>[2x]TLQPTEAAYIAGFLDGDGSIYARLEPRPDYKDIKYQVRLAISFIQRKDKFPYLQDIYDQLGKRGILRKDRGDGIADYRIYGSTHLSIILPDLVPYLRIKKKQANRI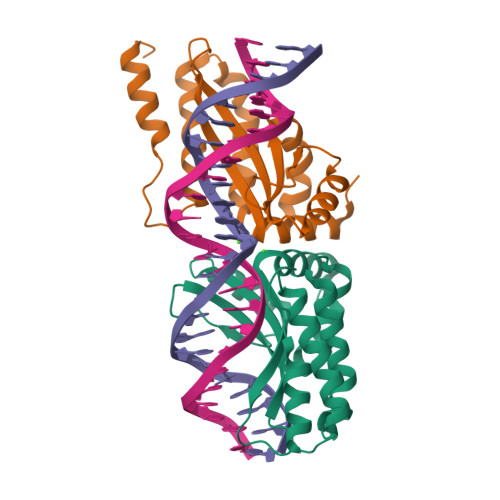LHIINLYPQAQKNPSKFLDLVKIVDDVQNLNKRADELKSTNYDRLLEEFLKAGKI Enzymes of the vanillyl alcohol oxidase/p-cresol methyl hydroxylase (VAO/PCMH) superfamily are found across all kingdoms where they perform a range of metabolic functions. These flavoproteins share a conserved FAD-binding domain and a more variable substrate-binding domain that enables interactions with a range of substrates. One of these, the 4-phenol oxidases/dehydrogenases, catalyzes the oxidation of para-substituted phenolic compounds. A fundamental distinction is that the oxidases efficiently react with oxygen producing hydrogen peroxide whereas the dehydrogenases hardly react with oxygen and typically employ other proteins, such as cytochrome c, as acceptors.

We first prepared and studied the P151L mutant, intended to mimic the N5 environment typical of the oxidases. The result was clear-cut: P151L-VAD can use dioxygen as an effective substrate for flavin re-oxidation. Therefore, P151L-VAD can be regarded as a competent oxidase. P151L is even more rapidly reduced with a kred value of 339 s-1, which is 600-fold faster than in the wild-type enzyme. Interestingly, we also found that the P151L enzyme binds the substrate with 40-fold lower affinity than the wild type. While flavin reduction in P151L is much faster, the mutant binds the substrate less avidly than the wild-type protein. In general, the oxidase-active variants (P151L, P151G, P151I, P151V) all adopt the trans conformation that slightly shifts the amino acid at position 151 away from the flavin. The analysis revealed a consistent pattern: in the oxidase mutants, the 150-153 loop conformations create tunnels that lead to the flavin re side.

>[2x]MAAPLPEGVSAEAMSSALDRFARIVGADWVFTEDKITPYEDPYTISNDETEHRPYAAVAPASTEEVQEIVRVANEFGVPLWPVSRGKNFAYGGAAPVMSGTVVLDMNRMNRILEVNEEFGYALVEPGVSYFELYDYIQEKGLKLWIDVPDLGWGSVVGNALDHGIGYTPYGDHFAMQCGMEVVLPNGEVVRTGMGAMPGNNTWQLFKYGYGPYVDGIFSQSNFGVVTKMGIWLMPEPAGYRPYLITFENEDDIETVTERLRPLKVAGVIQNGATVRSLVLDAAITRTKSQYYDGDGPIPPSVAKTMMADLDLGMWNFCGALYGPPPVMDTLWTAIRDSFADIPGVKFYFPEDRRHKVDLLLHRAETMKGVPKLTEFNFLNWDGGGGHVGFSPVSPITGKDAIKQYNMVSSRVREYGFDYMGLLAIGWRDLHHVTVIVYDKTDPDERKKLDELFNILVDEAAAEGYGEYRTHIRYMDRIAKTYSWNDNALWKMHETIKDALDPNGILAPGKSGIWGKNRRKA> MTWLTKIVPDLRYRQTRADFRTAGNLHRKLIRLSSDLGEERIANPRQQSGLLFRIEETRNELYLLVQSHSPLRVDRLGPGYHGVQMRNLDPFLARLDKGSRVRYRIVASPTKRLGRSENNTQRLGLKEPPKKPREYTWALRGAAAEEWWHSRAAANGLELLSTYAQTLDDVRDPGTADRSRKIRHPAVRFDGEAVISDVDAVRHAVLNGIGRGKSYGCGLLSLALIEEGEHG;> MLSVALCFLVGGAIPSPPSFDVTIAPWLIARSRDVLAAPEMLGLRDVLIRSHELSDVEIPLPPGAAVLWRILALITARITGLDQPPNKNPKRKWQARRSQILSKGRLDPEAVDAYFADYSERFDLFHPERPWLQDPRLREECPKTSGVNKLAWGRTAGENQVWLGGHHHDLDPHPLDSAEAVWHLLATLGYGPSGMCTARVVRGRSERNVTAGPLRGTVSYHPLGRTLFESLILNIPYPGTGAADLAFWEQPELNDPLGLPEESAGLAGILRLDHFRHAVLLHPSPDGSHVVDAWVTWAWRERNISPELDPYLIYQTSKEGRVYPRPAEAERAIWRDLDALLHYGEDGNYRPTILDNCTPLAQVPQEVLDSLRLRAFGFDQDGQARDKQWFTATTPAVLRWLADRETDDNENARIVRRITLARKAAEALGRRLEKACKEAWKESNSPSSTSSGTNAKTETGVGPWVQHGMSRYWAKAEPVFWNIVYDRPAQGYTPGMAGPGNAFNLVALAAYDEVTGPYCERPRVAKVVERHRSTLFSNWTPKQDKEAA;>MTFVDIHAIQTLPYSNINRDDLGSPKTVVYGGKERTRVSSQSWKRAVRHEVEARLGDKAVRTRRIISEIAKRLRERGWDADLADAGARQVVLSVGKKSGIKLEKEKDSEAPATSVLFYLPVPAIDELAAIADEHRDAVAKEAAKKTPKGILPADRITEVLKSRNVSVNLFGRMLAELPSTEVDGAVQFAHAFTVHGTTVEVDFFTAVDDIPKENDHGSGHMNAGQFSAGTFYRYANVNLDRLVENTGDAQTARTAVAEFLRAFLSTVPSGKQNATAAMTLPDLV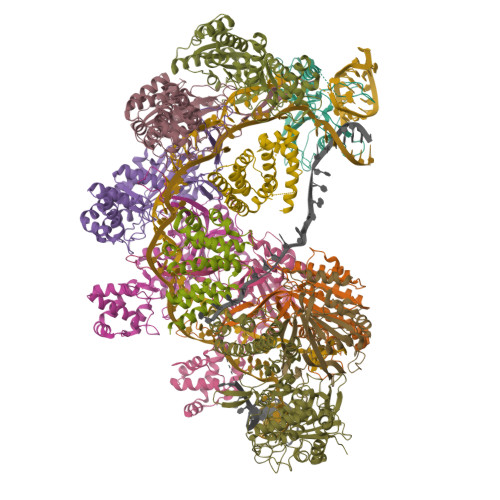HIAVRFDRPISFAPAFETALYGSDGYTLRACQELNNYAERLREVWPDDAIRGYATVENKTDLAALGERYDSYPALIDAMVAAAFEGERE[6x];>[2x]MNSDYILQHADALVKRVSKLIVNEPAARAALRRGVGLAPEDPRMLAAHRVVAPYVPVPTDYDVDRRRAASLWDVHAVERAFYAVAAIMAAQPRSARDQEAEATEEQTGEPQDSEALTEPTPAEESSATKDGKPDRRPNLGVSLAQAVFDKGLNADSTEQRLHLIARQNLDGVHRHLPRLVLYLRSDQVHIDWGILIRDLARWGHTPRHVAREWVQDYHRTLETLTRQAEQKNKNNTTDEEAEAA;> MSGFLLRLAGPMQSWGEHSMFGERDTLPYPSRSGLIGMFAAAQGVRRGDPLDRYKELKFTVRVDRPGVRLVDFHTIGGGLPKERTVPTAAGERRDPKKATIVTSRSYLADAVFTVAVTGPEADTIADALAAPYWQPYLGRRAFVPDPLLVLRRRVADPVRELVEAVPLPHRRVEEDAATVLVDLIYEEGEYPDTRTLTVLNDVPLSFDSKSRRYSTRQIRVVPTEVPATLVAGPGRDYQNKLFTYVKQCAEEAA>[2x]GGEQFTVKDNALTDDAIVPIKLSRTAEYIKDYLALKEIWDALNGKNWSQQGFGTQPGANWNFNKELDMWGAQPGVSLNSNGRVTGLSLEGFGASGRVPDAIGQLTELEVLALGSHGEKVNERLFGPKGISANMSDEQKQKMRMHYQKTFVDYDPREDFSDLIKDCINSDPQQKSIKKSSRITLKDTQIGQLSNNITFVSKAVMRLTKLRQFYMGNSPFVAENICEAWENENSEYAQQYKTEDLKWDNLKDLTDVEVYNCPNLTKLPTFLKALPEMQLINVACNRGISGEQLKDDWQALADAPVGEKIQIIYIGYNNLKTFPVETSLQKMKKLGMLECLYNQLEGKLPAFGSEIKLASLNLAYNQITEIPANFCGFTEQVENLSFAHNKLKYIPNIFDAKSVSVMSAIDFSYNEIGSVDGKNFDPLDPTPFKGINVSSINLSNNQISKFPKELFSTGSPLSSINLMGNMLTEIPKNSLKDENENFKNTYLLTSID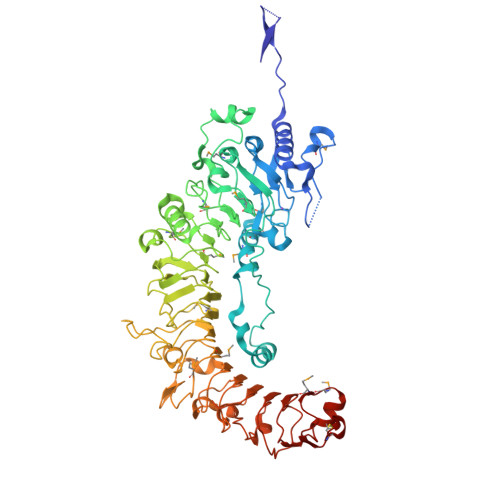LRFNKLTKLSDDFRATTLPYLVGIDLSYNSFSKFPTQPLNSSTLKGFGIRNQRDAQGNRTLREWPEGITLCPSLTQLQIGSNDIRKVNEKITPNISVLDIKDNPNISIDLSYVCPYIEAGMYMLFYDKTQDIRGCDALDIKR>MAHAGRTGYDNREIVMKYIHYKLSQRGYEWDAGDDVEENRTEAPEGTESEVVHLTLRQAGDDFSRRYRRDFAEMSSQLHLTPFTARGRFATVVEELFRDGVNWGRIVAFFEFGGVMCVESVNREMSPLVDNIALWMTEYLNRHLHTWIQDNGGWDAFVELYGPSM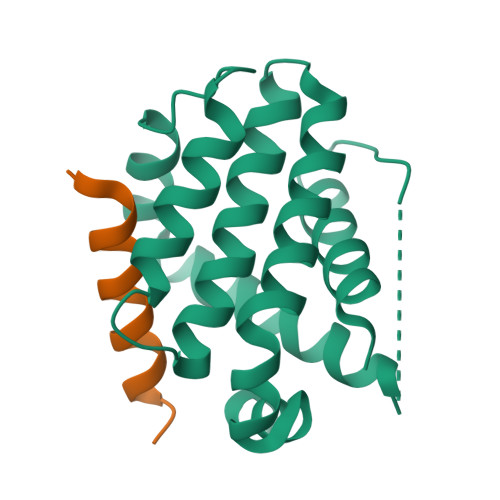R[2x];>[2x]HQAEVQIARKLQCIADQFHRLHVQQ>PEVVFGSMASRRSADPAKTLEAVSAVADWLRDPQRESPARAQLAEAVRLTARTLAAVAPGASVEVRVPPFVAVQCISGPKHTRGTPPNVVETDARTWLLLATG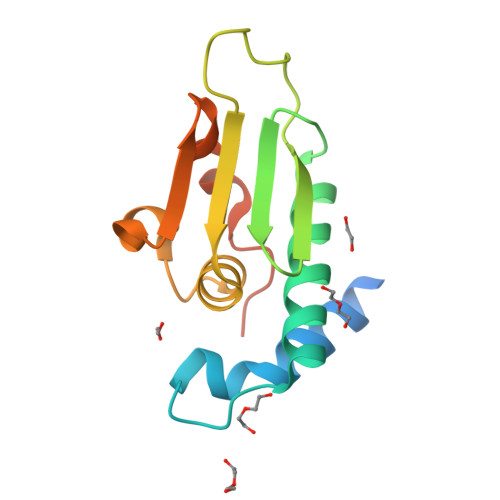LLDIADAGASVQMSGSRAAEVAHWLPVVRIDPSRHHHHHH[2x]>NAVESTLRRVAKDLTGLRQRWALVGGFAVSARSEPRFTRDVDIVVAVANDDAAESLVRQLLTQQYHLLASVEQDAARRLAAVRLGATADTAANVVVDLLFASCGIEPEIAEAAEEIEILPDL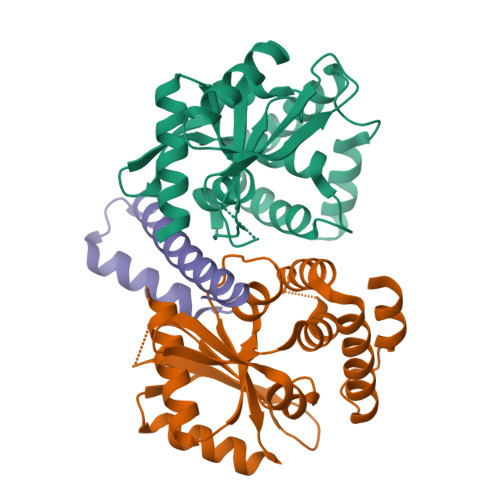VAPVATTAHLIAMKLLARDDDRRPQDRSDLRALVDAASPQDIQDARKAIELITLRGFHRDRDLAAEWTRLAAKW[2x];> AVSVAAQKLRLALDMYEVGEQMQRMRLGRERPNADVVEIEAAIDAWRMTRPGAEEGDSAGPTSTRFT TERT-BUTYL 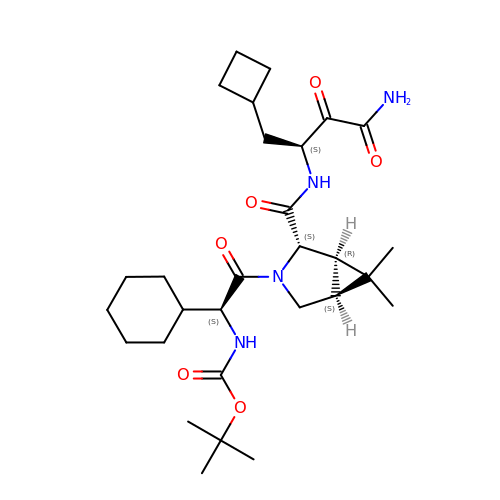{(1S)-2-[(1R,2S,5S)-2-({[(1S)-3-AMINO-1-(CYCLOBUTYLMETHYL)-2,3-DIOXOPROPYL]AMINO}CARBONYL)-6,6-DIMETHYL-3-AZABICYCLO[3.1.0]HEX-3-YL]-1-CYCLOHEXYL-2-OXOETHYL}CARBAMATE | C29 H46 N4 O6 | LFKITAOQQDIAJF-YFNVTMOMSA-N>GSH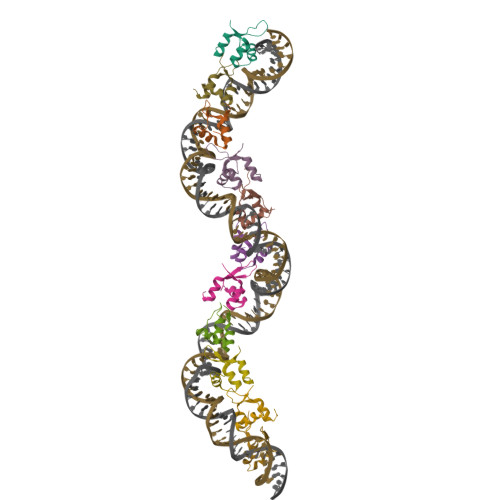MTARTPDAEPLLTPAEVATMFRVDPKTVTRWAKAGKLTSIRTLGGHRRYREAEVRALLAGIPQQRSEA[11x]>[6x]MGHHHHHHAIKKKDRIIGVKELEIPQELKLVPNWVLWRAEWNEKQQNFGKVPYSINGYRA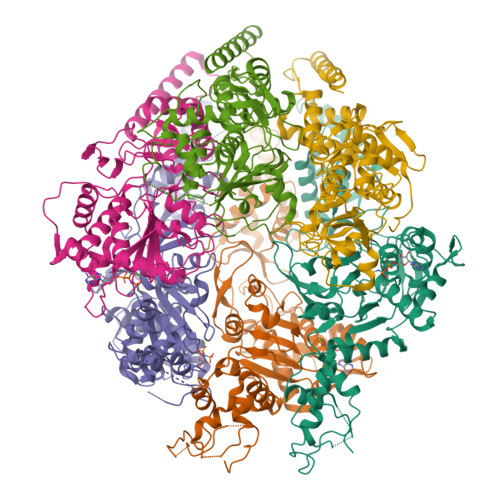STTNKKTWCDFESVSIEYEVDEQYSGIGFVLSDGNNFVCLDIDNAIDKKGQINSELALKMMQLTYCEKSPSGTGLHCFFKGKLPDNRKKKRTDLDIELYDSARFMTVTGCTIGQSDICDNQEVLNTLVDEYFKENLPANEVVREESNTNIQLSDEDIINIMMKSKQKDKIKDLLQGTYESYFESSSEAVQSLLHYLAFYTGKNKQQMERIFLNYNNLTDKWESKRGNTTWGQLELDKAIKNQKTIYTKSIDEFNVIPQGSKDVKQLLNQLGHEERTKMEENWIEEGKRGRKPTTISPIKCAYILNEHLTFILFDDEENTKLAMYQFDEGIYTQNTTIIKRVISYLEPKHNSNKADEVIYHLTNMVDIKEKTNSPYLIPVKNGVFNRKTKQLESFTPDYIFTSKIDTSYVRQDIVPEINGWNIDRWIEEIACNDNQVVKLLWQVINDSMNGNYTRKKAIFFVGDGNNGKGTFQELLSNVIGYSNIASLKVNEFDERFKLSVLEGKTAVIGDDVPVGVYVDDSSNFKSVVTGDPVLVEFKNKPLYRATFKCTVIQSTNGMPKFKDKTGGTLRRLLIVPFNANFNGIKENFKIKEDYIKNQQVLEYVLYKAINLDFETFDIPDASKKMLEVFKEDNDPVYGFKVNMFDQWTIRKVPKYIVYAFYKEYCDENGYNALSSNKFYKQFEHYLENYWKTDAQRRYDNEELAKRIYNFNDNRNYIEPIESGKNYKSYEKVKLKAI> ESAFNQTEFNKLLLECVVKTQSSVAKILGIESLSPHVSGNSKFEYANMVEDIREKVSSE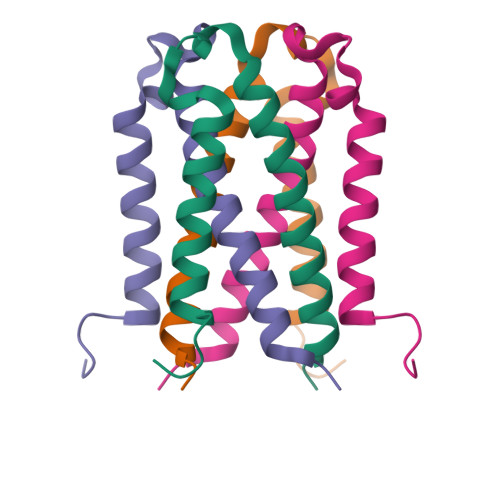MERFFPKNDDE> MHHHHHHIFPKQYPIINFTTAGATVQSYTNFIRAVRGRLTTGADVRHEIPVLPNRVGLPINQRFILVELSNHAELSVTLALDVTNAYVVGYRAGNSAYFFHPDNQEDAEAITHLFTDVQNRYTFAFGGNYDRLEQLAGNLRENIELGNGPLEEAISALYYYSTGGTQLPTLARSFIICIQMISEAARFQYIEGEMRTRIRYNRRSAPDPSVITLENSWGRLSTAIQESNQGAFASPIQLQRRNGSKFSVYDVS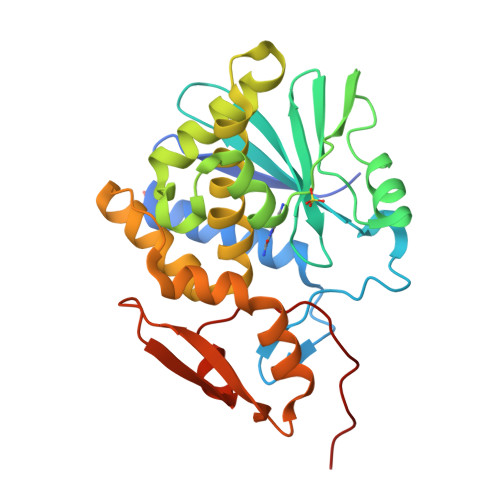ILIPIIALMVYRCAPPPSSQF>[4x]SHMERVFVWDLDETIIIFHSLLTGTFASRYGKDTTTSVRIGLMMEEMIFNLADTHLFFNDLEDCDQIHVDDVSSDDNGQDLSTYNFSADGFHSSAPGANLCLGSGVHGGVDWMRKLAFRYRRVKEMYNTYKNNVGGLIGTPKRETWLQLRAELEALTDLWLTHSLKALNLINSRPNCVNVLVTT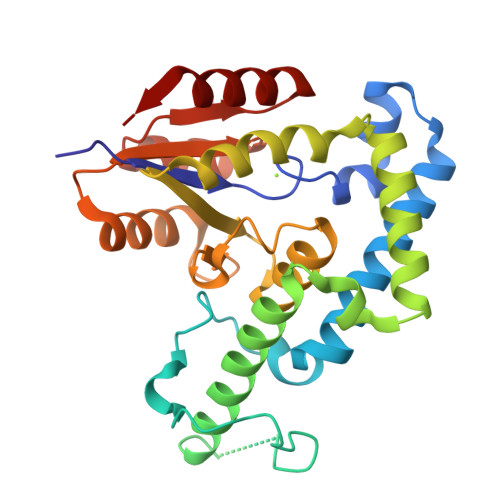TQLIPALAKVLLYGLGSVFPIENIYSATKTGKESCFERIMQRFGRKAVYVVIGDGVEEEQGAKKHNMPFWRISCHADLEALRHALELEYL> EESEERD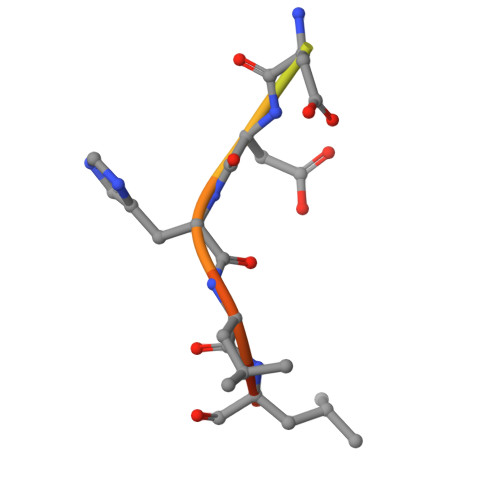DHLLPM> IRYVVIDIETDGKDAKRNHILEIGAIRCEDGKE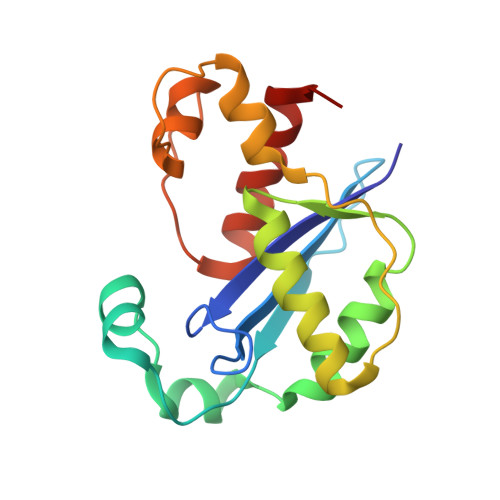THFTALISGDAVPPSITKLTGITATLLQKEGQEEKKVLTAFREFIGDDDLVGYHVSFDIEFLRQAFKKYGLGYLKNKTHDLLRIVKKEQLFQADYKLETSLQSYGIHKKVPHRALGDAELVKCLAKKLNKF> KVTMNDFDYLKLLGKGTFGKVILVREKATGRYYAMKILRKEVIIAKDEVAHTVTESRVLQNTRHPFLTALKYAFQTHDRLCFVMEYANGGELFFHLSRERVFTEERARFYGAEIVSALE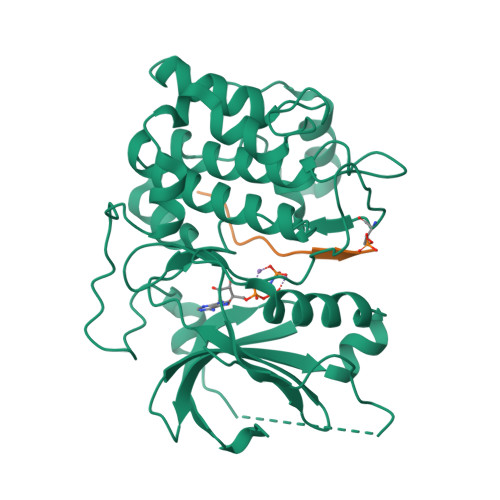YLHSRDVVYRDIKLENLMLDKDGHIKITDFGLCKEGISDGATMKTFCGTPEYLAPEVLEDNDYGRAVDWWGLGVVMYEMMCGRLPFYNQDHERLFELILMEEIRFPRTLSPEAKSLLAGLLKKDPKQRLGGGPSDAKEVMEHRFFLSINWQDVVQKKLLPPFKPQVTSEVDTRYFDDEFTAQSITITPPDRYDSLGLLELDQRTHFPQFDYSASIRE;> GRPRTTSFAE>[72x]XL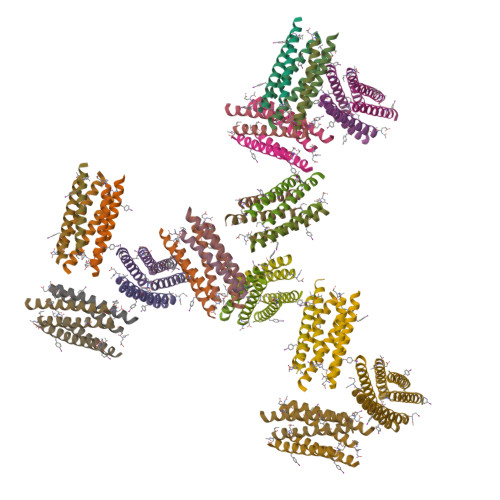KAIAQEFKAIAKKFKAIAFEFKAIAQKX>[6x]MFEARLVQGSILKKVLEALKDLINEACWDISSSGVNLQSMDSSHVSLVQLTLRSEGFDTYRCDRNLAMGVNLTSMSKILKCAGNEDIITLRAEDNADTLALVFEAPNQEKVSDYEMKLMD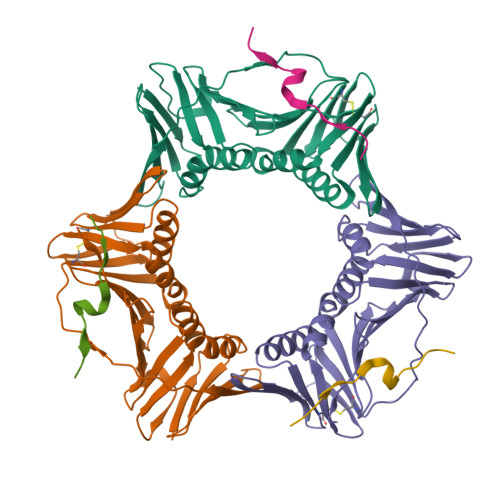LDVEQLGIPEQEYSCVVKMPSGEFARICRDLSHIGDAVVISCAKDGVKFSASGELGNGNIKLSQTSNVDKEEEAVTIEMNEPVQLTFALRYLNFFTKATPLSSTVTLSMSADVPLVVEYKIADMGHLKYYLAPKIEDEEGS;>SAVLQKKITDYFHPKK[6x]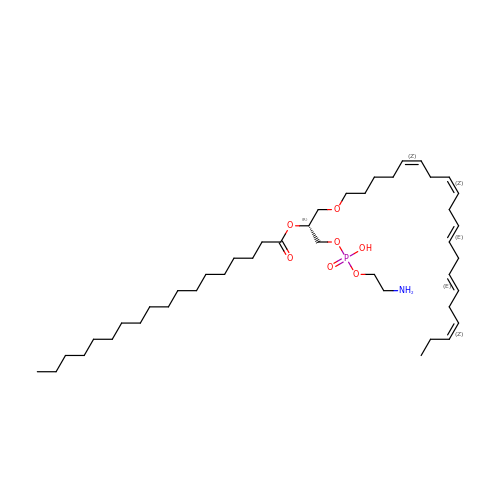[(2~{R})-1-[2-azanylethoxy(oxidanyl)phosphoryl]oxy-3-[(5~{Z},8~{Z},11~{E},14~{E},17~{Z})-icosa-5,8,11,14,17-pentaenoxy]propan-2-yl] octadecanoate | C43 H78 N O7 P | BCVRSQNGADAZKS-GZACMAKJSA-N>[2x]APISLPAGTYTLKNVSTGTVLDLWRGEAAEGTAIQGYKSHGGDNQKWRLKWTGKGNQVTLQNVKSGTYVGTASNIQNSVN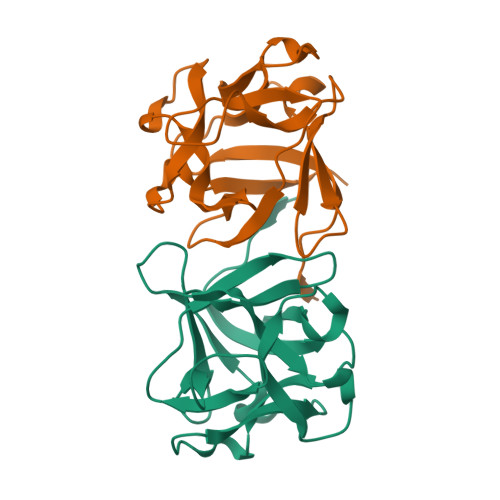VVGSTTAVPLDIVAADKGFAIEAADHRLFVLDLKESNPANETPVIYYNNNATDNQKWKFIDEK> HGMSQPACTARRRTRVLILGVNGFIGNHLTERLLREDHYEVYGLDIGSDAISRFLNHPHFHFVEGDISIHSEWIEYHVKKCDVVLPLVAIATPIEYTRNPLRVFELDFEENLRIIRYCVKYRKRIIFPSTSEVYGMCSDKYFDEDHSNLIVGPVNKPRWIYSVSKQLLDRVIWAYGEKEGLQFTLFRPFNWMGPRLDNLNAARIGSSRAITQLILNLVEGSPIKLIDGGKQKRCFTDIRDGIEALYRIIENAGNRCDGEIINIGNPENEASIEELGEMLLASFEKHPLRHHFPPFAGFRVVESSSYYGKGYQDVEHEKPSIRNAHRCLDW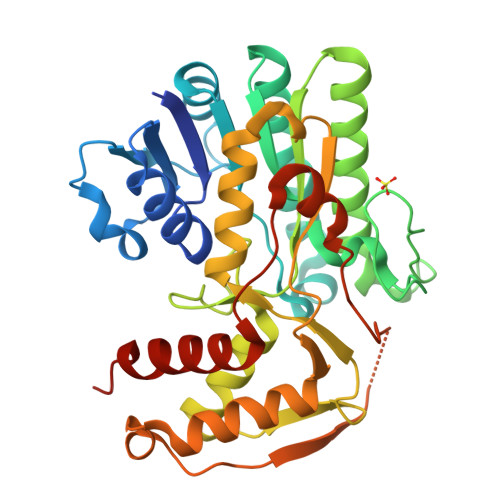EPKIDMQETIDETLDFFLRTVDLTDKPS>GPAAAPALDTLPAPTSLVLSQVTSSSIRLSWTPAPRHPLKYLIVWRASRGGTPREVVVEGPAASTEL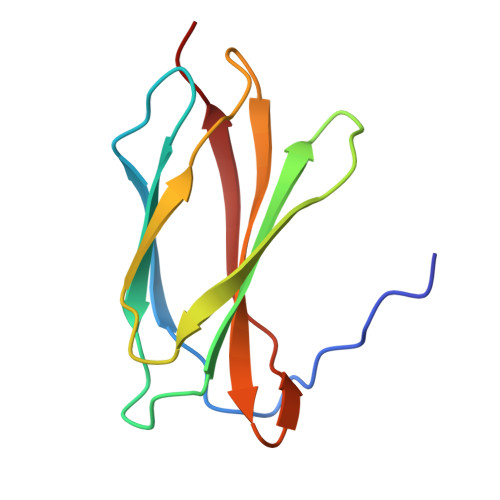HNLASRTEYLVSVFPIYEGGVGEGLRGLVTTAP[4x]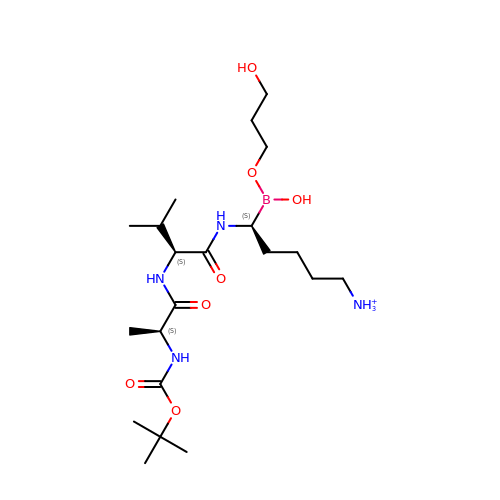N-(tert-butoxycarbonyl)-L-alanyl-N-{(1S)-5-ammonio-1-[hydroxy(3-hydroxypropoxy)boranyl]pentyl}-L-valinamide | C21 H44 B N4 O7 | JPOFXBAJTXFLAJ-ULQDDVLXSA-O> MNRFFKVSSKYQYYKYLEQYDAAFLRKYQSETHWYLGRRGAWKNLVIKYAGDHISLEEEHNVKYKTHLSFVYLSYRL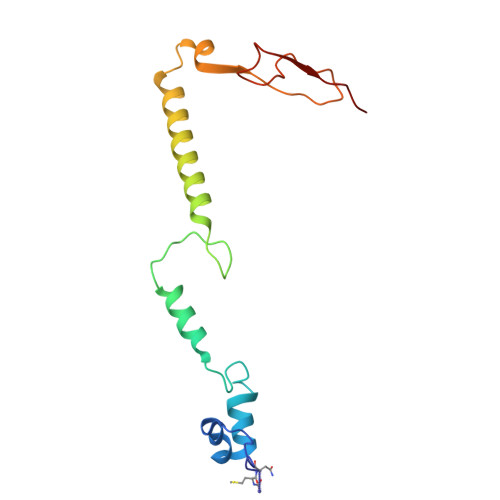AWVLFAYVLIYNHFLLGDIGKTFNVGEWDHRLKPSAERDYPTRYESLYILDRTQKW> MANFVIPYLKPVADFWNSLCIDQHQDSLFQFKGQTGSLGTDWTSKYLRSEQDVYNHKYLQYHKRVHEAPELTDVISDNVYRLTLFAGVERVLSVRQAQAILKTQFAGATENISGAFQTVLNGGIFRRGYFRGALLNLLQFCGAPYQSLIWSRNSGITNQVIVSSIFEAFFYPLDTVKTLIYNDVQGKYKGAFHCASQVVQNAGWSRLYA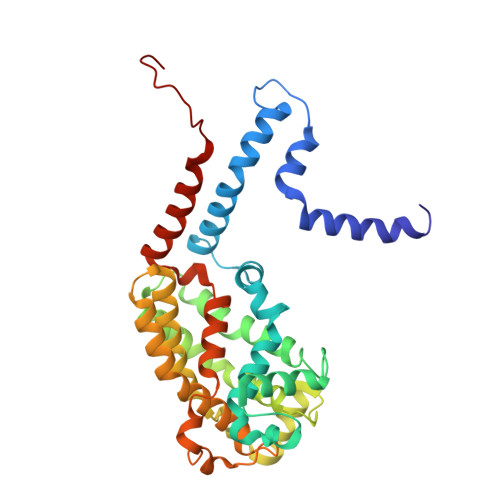GIFQKLIFNSALIFHLNQVWDGSSQQWASLALVAAAYPLLVLKTRFQVAGTPLALATSNEVLKVNRKTLYAGLVPYLIFNTLFAYEFAAWHSSTAQERVIGGLQNAMKQFSSPAAEQVWSS Glycan uptake across the bacterial outer membrane (OM) of these bacteria is mediated by SusCD protein complexes, comprising a membrane-embedded barrel and a lipoprotein lid, that is thought to open and close to facilitate substrate binding and transport. Here we show that for both the levan and dextran utilisation systems of Bacteroides thetaiotaomicron, the additional OM components assemble on the core SusCD transporter, forming stable glycan utilising machines which we term ‘utilisomes’. Transport-competent FOS are generated from levan by a surface-exposed lipoprotein, a GH32-family levan endo-glycanase (GHlev), while an SGBP (SGBPlev) is thought to recruit levan at the cell surface. Single particle cryogenic electron microscopy (cryoEM) structures in the absence and presence of substrate reveal concerted conformational changes that demonstrate the mechanism of substrate capture, and rationalise the role of each component in the utilisome.

Upon addition of substrate, the levan utilisome undergoes large conformational changes, revealing the substrate-bound states of GHlev and SGBPlev, and demonstrating that the pedal-bin mechanism of nutrient capture operates in the presence of all OM-localised components of the PUL. The resulting 3D structure reveals that FOS binding drives major conformational change in the utilisome. All SusDlev lids are closed, tightly capping the extracellular face of the SusClev barrels, relative to the open position in the apo utilisomes. 3D classification reveals that the major source of heterogeneity present in the data was the presence of sub-complexes missing one or more accessory lipoproteins (ED Fig. 3b), so to probe substrate binding within the closed transporter complex, we first performed targeted refinement of the SusCDlev core, using particle subtraction to remove the signal for GHlev and SGBPlev from the images. (3) Binding of the oligosaccharide to SusCD promotes lid closure and signalling to the plug, breaks the aromatic lock and exposes the Ton box to the periplasm.

>[2x]MPGIMKNKKLLCSVCFLFAFMSALWGQNITVKGNVTSKTDGQPIIGASVVETTATTNGTITDFDGNFTLSVPVNSTLKITYIGYKPVTVKAAAIVNVLLEEDTQMVDEVVVTGYTTQRKADLTGAVSVVKVDEIQKQGENNPVKALQGRVPGMNITADGNPSGSATVRIRGIGTLNNNDPLYIIDGVPTKAGMHELNGNDIESIQVLKDAASASIYGSRAANGVIIITTKQGKKGQIKINFDASVSASMYQSKMNVLNTEQYGRAMWQAYVNDGENPNGNALGYAYNWGYNADGNPVLYGMTLSKYLDSKNTMPVADTDWFDEITRTGVIQQYNLSVSNGSEKGSSFFSLGYYKNLGVIKDTDFDRFSARMNSDYKLIDDILTIGQHFTLNRTSEVQAPGGIIETALDIPSAIPVYASDGSWGGPVGGWPDRRNPRAVLEYNKDNRYTYWRMFGDAYVNLTPFKGFNLRSTFGLDYANKQARYFTYPYQEGTQTNNGKSAVEAKQEHWTKWMWNAIATYQLEVGKHRGDVMIGMELNREDDSHFSGYKEDFSILTPDYMWPDAGSGTAQAYGAGEGYSLVSFFGKMNYSYADRYLLSLTLRRDGSSRFGKNHRYATFPSVSLGWRITQENFMKELTWLDDLKLRASWGQTGNQEISNLARYTIYAPNYGTTDSFGGQSYGTAYDITGSNGGGVLPSGFKRNQIGNDNIKWETTTQTNVGIDFSLFKQSLYGSLEYYYKKATDILTEMAGVGVLGEGGSRWINSGAMKNQGFEFNLGYRNKTAFGLTYDLNGNISTYRNEILELPETVAANGKFGGNGVKSVVGHTYGAQVGYIADGIFKSQDEVDNHATQEGAAVGRIRYRDIDHNGVIDERDQNWIYDPTPSFSYGLNIYLEYKNFDLTMFWQGVQGVDIISDVKKKSDFWSASNVGFLNKGTRLLNAWSPTNPNSDIPALTRSDTNNEQRVSTYFVENGSFLKLRNIQLGYTVPAVISKKMRMDRLRFYCSAQNLLTIKSKNFTGEDPENPNFSYPIPVNITFGLNIGF;>MKKIIYIATIGITLLTTSCDDFLDRQVPQGIVTGDQIASPEYVDNLVISAYAIWATGDDINSSFSLWNYDVRSDDCYKGGSGTEDGGVFNALEISKGINTTDWNINDIWKRLYQCITRANTALQSLDQMDEKTYPLKNQRIAEMRFLRGHAHFMLKQLFKKIVIVNDENMEPDAYNELSNTTYTNDEQWQKIADDFQFAYDNLPEVQIEKGRPAQAAAAAYLAKTYLYKAYRQDGADNALTGINEEDLKQVVKYTDPLIMAKGGYGLETDYSMNFLPQYENGAESVWAIQYSINDGTYNGNLNWGMGLTTPQILGCCDFHKPSQNLVNAFKTDSQGKPLFSTYDNENYEVATDNVDPRLFHTVGMPGFPYKYNEGYIIQKNDDWSRSKGLYGYYVSLKENVDPDCDCLKKGSYWASSLNHIVIRYADVLLMRAEALIQLNDGRITDAISLINEVRSRAAGSTMLIFNYKEDYGVNFKVTPYDLKAYAQDEAMKMLKWERRVEFGMESSRFFDLVRWGEAKDVINAYYVTEASRCSIYKNAGFTENKNEYLPVPFEQISASNGNYTQNFGWAAAAHHHHHH[2x];>[2x]MMKNMILPIAFTALIASMTACSDETDPILTQKNWDGTATYFQSSDEHGFSMYYKPQVGFVGDPMPFYDPVAKDFKVMYLQDYRPNPEATYHPIFGVATKDGATYESLGELISCGGRDEQDAAIGTGGTIYNPADKLYYTFYTGNKFKPSSDQNAQVVMVATSPDFKTWTKNRTFYLKGDTYGYDKNDFRDPFLFQTEDGVYHMLIATRKNGKGHIAEFTSADLKEWESAGTFMTMMWDRFYECPDVFKMGDWWYLIYSEQASFMRKVQYFKGRTLEDLKATTANDAGIWPDNREGMLDSRAFYAGKTASDGTNRYIWGWCPTRAGNDNGNVGDVEPEWAGNLVAQRLIQHEDGTLTLGVPDAIDRKYTSAQEVKVMAKDGNMIESGKTYTLGEGASVIFNRLKVHNKISFTVKTASNTDRFGISFVRGTDSASWYSIHVNADEGKANFEKDGDDAKYLFDNKFNIPADNEYRVTIYSDQSVCVTYINDQLSFTNRIYQMQKNPWSLCCYKGEITVSDVQVSTY;>MKSIIKQLYTILLVTVACLTVTGCSDDFKSGLRLDGDVWVNSIRLDEYAGTVDYQNKAIVVGVPYDYDITRMVVTEMNLSEGAKASIAIGETIDFSLPVSLTVKNGDVQMSYTITVKRDEAKILTFKLNDTYVGKVDQLSKTISVVVPLTVDITQLKGTFTVTDGATVTPASGSIQDFTNPVTYTATYRSAVTPYVVTVTQGNVIPTAFVGTASSVSLLTSPEEKAAAQWMMDNVSMSEYISFKDVVDGKVDLGKYTAIWWHFHADNGDNPPLPDDAKAAAEKFKVYYQNGGNLLLTRYATFYIANLGIAKDERVPNNSWGGNEDSPEITSAPWSFLITGSESHPLFQDLRWKDGDKSTVYTCDAGYAITNSTAQWHIGTDWGGYDDLNAWRNLTGGIDLAHGGDGAVVIAEFEPRSNSGRTLCIGSGCYDWYGKGVDASADYYHYNVEQMTLNAINYLCK[2x]> KQLA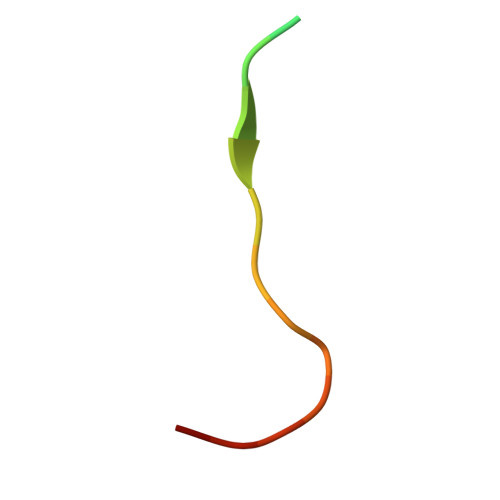TKAARKSAPATGGVK> MTSPQLEWTLQTLLEQLNEDELKSFKSLLWAFPLEDVLQKTPWSEVEEADGKKLAEILVNTSSENWIRNATVNILEEMNLTELCKMAKAEMMEDGQVQEIDNPELGDAEEDSELAKPGEKEGWRNSMEKQSLVWKNTFWQGDIDNFHDDVTLRNQRFIPFLNPRTPRKLTPYTVVLHGPAGVGKTTLAKKCMLDWTDCNLSPTLRYAFYLSCKELSRMGPCSFAELISKDWPELQDDIPSILAQAQRILFVVDGLDELKVPPGALIQDICGDWEKKKPVPVLLGSLLKRKMLPRAALLVTTRPRALRDLQLLAQQPIYVRVEGFLEEDRRAYFLRHFGDEDQAMRAFELMRSNAALFQLGSAPAVCWIVCTTLKLQMEKGEDPVPTCLTRTGLFLRFLCSRFPQGAQLRGALRTLSLLAAQGLWAQMSVFHREDLERLGVQESDLRLFLDGDILRQDRVSKGCYSFIHLSFQQFLTALFYALEKEEGEDRDGHAWDIGDVQKLLSGEERLKNPDLIQVGHFLFGLANEKRAKELEATFGCRMSPDIKQELLQCKAHLHANKPLSVTDLKEVLGCLYESQEEELAKVVVAPFKEISIHLTNTSEVMHCSFSLKHCQDLQKLSLQVAKGVFLENYMDFELDIEFERCTYLTIPNWARQDLRSLRLWTDFCSLFSSNSNLKFLEVKQSFLSDSSVRILCDHVTRSTCHLQKVEIKNVTPDTAYRDFCLAFIGKKTLTHLTLAGHIEWERTMMLMLCDLLRNHKCNLQYLRLGGHCATPEQWAEFFYVLKANQSLKHLRLSANVLLDEGAMLLYKTMTRPKHFLQMLSLENCRLTEASCKDLAAVLVVSKKLTHLCLAKNPIGDTGVKFLCEGLSYPDCKLQTLVLQQCSITKLGCRYLSEALQEACSLTNLDLSINQIARGLWILCQALENPNCNLKHLRLWSCSLMPFYCQHLGSALLSNQKLETLDLGQNHLWKSGIIKLFGVLRQRTGSLKILRLKTYETNLEIKKLLEEVKEKNPKLTIDC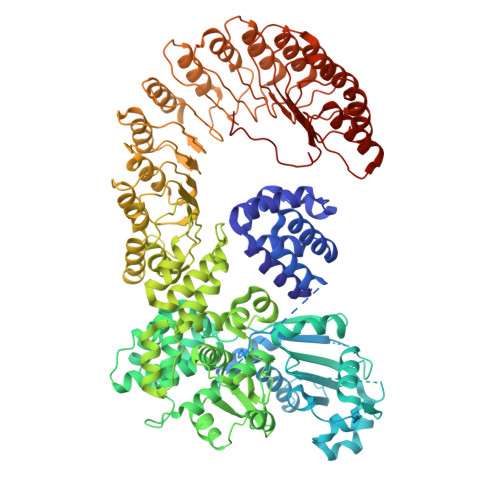NASGATAPPCCDFFC> DYKLFITEGYEVGRVNGLAVIGESAGIVLPIIAEVTPSMSKSEGRVIATGRLQEIAREAVMNVSAIIKKYTGRDISNMDVHIQFVGTYEGVEGASASISIATAVISAIEGIPVDQSVAMT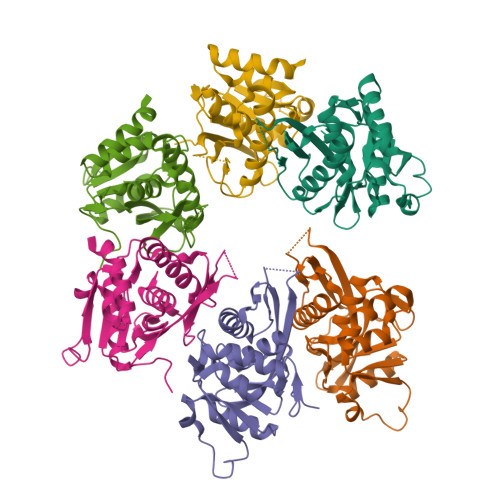GSLSVKGEVLPVGGVTQKIEAAIQAGLKKVIIPKDNIDDVLLDAEHEGKIEVIPVSRINEVLEHVLEDGKKKNRLMSKFKELELAAV>ETGCPANCLCSKTDINCKKPDDGNLFPLLEGQDSRNITSIHIENWKNLQTLNAVDMELYTGLQRLTIRNSGLRNIQPRAFAKNPHLRYIDLSGNRLTTLSWQLFQTLRLFDLRLERNPFQCSCDIRWIQLWQEKGEANLQSQQLHCMNLDTAVILLRNMNITQCDLPEISVSHVNLTVREGENAVITCQGSGSPLPDVDWTVADLHSINTHQTNLQWTNVHAIQLTLVNVTSEDNGFLLTCIAENVVGMSQASVLLTVYGTKHHHHHH[2x];>ETGESPPVFIKKPVDQIGVSGGVASFVCQATGDPKPRVTWNKKGKKVNSQRFETIEFDESAGAVLRIQPLRTPRDENIYECVAQNPHGEVTVHAKLTVLREDQLPPGFPNIDMGPQLKVVERTRTATMLCAASGNPDPEITWFKDFLPVDPSTSNGRIKQLRSGGLQIESSEETDQGKYECVASNSAGVRYSSPANLYVRVRRVAPRFSILPVSHEIMPGGNVNITCVAVGSPMPYVKWMQGAEDLTPEDDMPVGRNVLELTDVKDSANYTCVAMSSLGVIEAVAQITVKSKGHHHHHH[3x]

At the axonal surface, type IIa receptor protein tyrosine phosphatases (RPTPs) (type IIa RPTPs, for example, RPTPσ, RPTPδ and leukocyte common antigen-related (LAR) in vertebrates, dLAR in Drosophila), are a recently identified nexus for extracellular interactions, receiving signals and transmitting them intracellularly to the cytoskeleton to regulate neuronal extension and guidance, as well as synaptic organization. There are two major neuronal RPTPσ isoforms, sharing a common intracellular catalytic region and an extracellular region predicted to contain three immunoglobulin (Ig)-like domains followed by either five or nine fibronectin (FN) type III domains, in the central and peripheral nervous systems, respectively. Previous mutagenesis and structural studies have demonstrated that the proteoglycan-binding site lies on Ig1 of RPTPσ, and comprises an extended positively charged surface of basic residues101314. Binding of postsynaptic TrkC, is reported to require the N-terminal three Ig domains of RPTPσ17; the NGL-3-binding site has been mapped to the FN1-2 domains.

To facilitate crystallization, a chicken TrkC construct (TrkC LRRIg1cryst) was generated, which removed putative sites of N-linked glycosylation and residues 63–77, a predicted disordered loop. A 2.5Å crystal structure of a chicken RPTPσ Ig1–2:TrkC LRRIg1cryst complex was determined, revealing a 1:1 stoichiometry, in agreement with results from multi-angle light scattering (MALS) analysis. The structure is consistent with a trans RPTPσ:TrkC complex spanning the synaptic cleft. The V-shaped RPTPσ Ig1–2 module contacts an extended TrkC surface consisting of the LRR convex face and Ig1 domain, with a buried surface area of 1,093 Å2 per molecule. Three major contact sites constitute the protein–protein interface in the complex crystal structure: site 1, RPTPσ Ig1:TrkC Ig1; site 2, RPTPσ Ig1:TrkC LRRIg1 inter-domain region and site 3, RPTPσ Ig2:TrkC LRR. Electrostatic interactions involving RPTPσ residues R96 and R99 and TrkC residues D240 and D242 dominate interactions at site 1. At site 2, Q75 in RPTPσ, interacts with TrkC residues E287 and Q148, while the side chains of RPTPσ E78 and TrkC R121 form a salt bridge. Site 3 centres on a K203–E100 salt bridge between RPTPσ and TrkC residues, respectively. RPTPσ:TrkC crystal structures provide an explanation for the specificity of this interaction and also highlight an overlap of TrkC and proteoglycan-binding sites on RPTPσ.> SN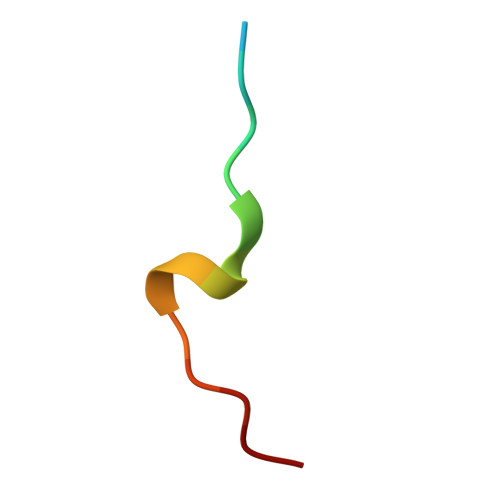SHQNVLSNYFPRVS>[2x]GEVVDCHLSDMLQQLHSVNASKPSERGLVRQEEAEDPACIPIFWVSKWVDYSDKYGLGYQLCDNSVGVLFNDSTRLILYNDGDSLQYIERDGTESYLTVSS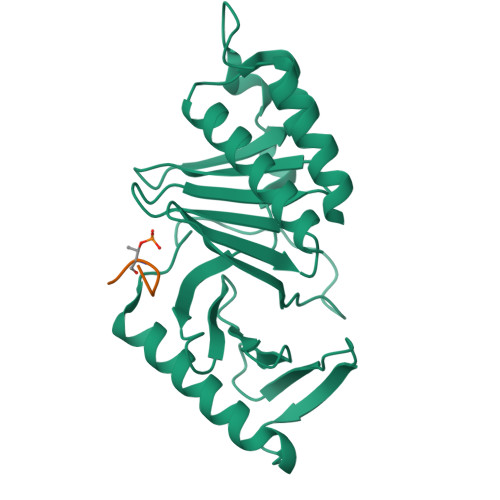HPNSLMKKITLLKYFRNYMSEHLLKAGANITPREGDELARLPYLRTWFRTRSAIILHLSNGSVQINFFQDHTKLILCPLMAAVTYIDEKRDFRTYRLSLLEEYGCCKELASRLRYARTMVDKLLSSRSASNRLKAS;>[2x]PMQSTPL Mounting evidence indicates that CRISPR and Cas proteins represent a microbial immune system that protects against invading foreign genetic elements, such as plasmids and phages. Csn2 is one of four Cas proteins that comprise the Nmeni subtype of the CRISPR/Cas system. The results of the mobility shift assay indicate that S. pyogenes Csn2 has a non-specific dsDNA-binding function. The tetrameric nature of S. pyogenes Csn2 results in a diamond-shaped ring structure with a positively charged inner surface as seen in E. faecalis Csn2.

The crystal structure of S. pyogenes Csn2 was determined to a resolution of 2.2 Å using multiwavelength anomalous diffraction. The asymmetric unit of the structure contains two S. pyogenes Csn2 monomers, three calcium ions, 204 water molecules and two ethylene glycol molecules. The monomeric structure of S. pyogenes Csn2 contains six α-helices (α1–α6) and nine β-strands (β1–β9), and is organized into two domains. In the asymmetric unit, the two S. pyogenes Csn2 monomers form a dimer with approximate two-fold non-crystallographic symmetry. The close proximity of the α-helical domains of the two symmetry-related dimers indicates dimerization of the dimers, resulting in a S. pyogenes Csn2 tetramer. Six calcium ions (four in CA1 sites and two in CA2 sites) are present in the S. pyogenes Csn2 tetramer, compared with eight calcium ions per E. faecalis Csn2 tetramer. The only CA2 site in the asymmetric unit of the S. pyogenes Csn2 structure is located adjacent to one of the two hinge regions in monomer A. The calcium ion in the CA2 site is coordinated by three residues (Glu138, Asp142, and Glu150) from monomer A, Asp118 from monomer B of the symmetry-related dimer, and two water molecules. In the corresponding hinge region of monomer B in the asymmetric unit, we were unable to locate a calcium ion. Residues in the hinge region of monomer A are structurally stabilized by the calcium ion bound in the nearby CA2 site, which is missing in monomer B. Such heterogeneity suggests that calcium binding in S. pyogenes Csn2 is important not only for its oligomerization, but also for its conformational diversity, enabling calcium-dependent conformational changes in the protein. However, the results of the metal analysis support full calcium ion occupancy in the CA1 sites of the selenomethionyl Csn2 protein used to determine the crystal structure.

>[2x]GSFTMNLNFSLLDEPIPLRGGTILVLEDVCVFSKIVQYCYQYEEDSELKFFDHKMKTIKESEIMLVTDILGFDVNSSTILKLIHADLESQFNEKPEVKSMIDKLVATITELIVFECLENELDLEYDEITILELIKSLGVKVETQSDTIFEKCLEILQIFKYLTKKKLLIFVNSGAFLTKDEVASLQEYISLTNLTVLFLEPRELYDFPQYILDEDYFLITKNMV> MGSSHHHHHHSSGLVPRGSHMSPSPVPGSQNVPA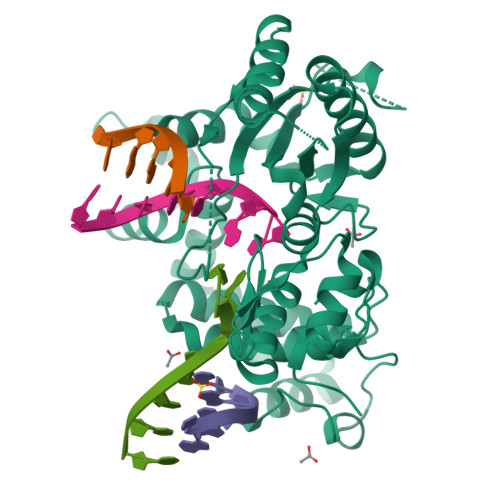PAVKKISQYACQRRTTLNNYNQLFTDALDILAENDELRENEGSCLAFMRASSVLKSLPFPITSMKDTEGIPCLGDKVKSIIEGIIEDGESSEAKAVLNDERYKSFKLFTSVFGVGLKTAEKWFRMGFRTLSKIQSDKSLRFTQMQKAGFLYYEDLVSCVNRPEAEAVSMLVKEAVVTFLPDALVTMTGGFRRGKMTGHDVDFLITSPEATEDEEQQLLHKVTDFWKQQGLLLYCDILESTFEKFKQPSRKVDALDHFQKCFLILKLDHGRVHSEKSGQQEGKGWKAIRVDLVMCPYDRRAFALLGWTGSRQFERDLRRYATHERKMMLDNHALYDRTKRVFLEAESEEEIFAHLGLDYIEPWERNA>[2x]MSLSKSLQKPTILNVETVARSRLFTVESVDLEFSNGVRRVYERMRPTNREAVMIVPIVDDHLILIREYAVGTESYELGFSKGLIDPGESVYEAANRELKEEVGFGANDLT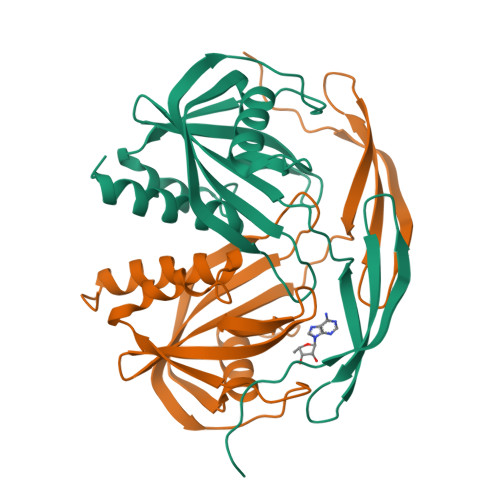FLKKLSMAPSYFSSKMNIVVAQDLYPESLEGDEPEPLPQVRWPLAHMMDLLEDPDFNEARNVSALFLVREWLKGQGRVEGGSHHHHHH>[4x]GSRQIVDAQAVCTRCKESADFWCFECEQLLCAKCFEAHQWFLKHEARPLAE

The ProMyelocyticLeukemia (PML) protein, also known as TRIM19, is the core component of PML nuclear bodies (NBs) that are tightly associated with nuclear matrix. It has been reported that PML NB can play many instrumental roles in DNA-damage responses, apoptosis, cellular senescence, and angiogenesis, etc. Previous studies have shown that the integrity of RBCC domain is essential for PML NB formation. In this study, we also report a previously unrecognized B1-box polymerization (n > 4) that is essential for PML/TRIM19 nuclear body assembly.

In line with the GF/UC analysis above, the structure of B1-box was determined to 2.0 Å resolution, unveiling an unexpected oligomerization in PML. In the B1-box monomer, the residues 120–127 fold into a loop-like subdomain 1 (SD1), which is ~12 Å away from the B1 core. In comparison, the residues 128–167, coordinated by two Zn ions, fold into a compact global domain, termed subdomain 2 (SD2). The subdomain 2 is a typical B-box-type Zn finger fold with a conserved β1–β2–α1–β3 arrangement and Zn-binding residues. The α1 helix and β-sheet are coordinated with two Zn ions, residues C129/C132/C148/C151 (Zn1) and C140/C143/H155/H161 (Zn2). In W157-dimer, the inter-molecular engagement is mainly mediated by two sets of hydrophobic interactions between W157 and F152/F138. In F158-dimer, the bulky hydrophobic side-chains are located in the heart of the dimeric interface, reminiscent of L73–L73 handshake in PML RING dimerization. In SD1-dimer, the N-terminal I122 and V123 residues could undergo a loop-to-strand transition to seal two B1s together via β-strand augmentation. The intermittent engagement between W157- and F158-interfaces enables the formation of a “brick”-like tetramer. In the α1-mediated W-shape coiled-coil, the K160 residues are consistently placed at the bottom of the B1 tetramer, giving rise to a highly concentrated Lys patch/lining.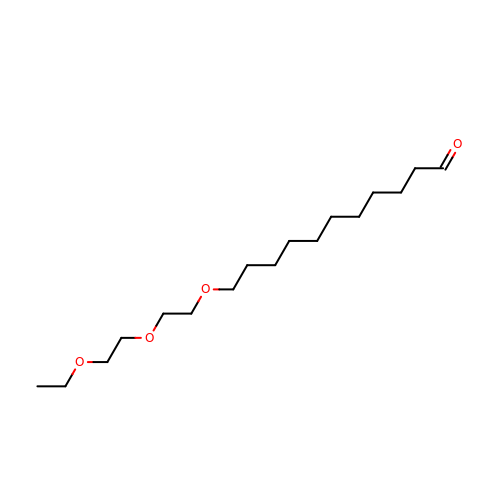11-[2-(2-ethoxyethoxy)ethoxy]undecanal | C17 H34 O4 | FUVMRIQNBOWRMW-UHFFFAOYSA-N{(2R)-4-[hydroxy(methyl)amino]-4-oxo-2-phenylbutyl}phosphonic 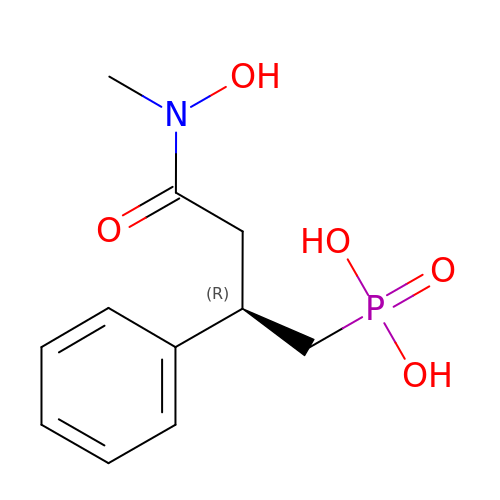acid | C11 H16 N O5 P | RGWBBKVQKPJVGW-JTQLQIEISA-N>GLEALLRPKSIAVIGASMKPNRAGYLMMRNLLAGGFNGPVLPVTPAWKAVLGVLAWPDIASLPFTPDLAVLCTNASRNLALLEELGEKGCKTCIILSAPASQHEDLRACALRHNMRLLGPNSLGLLAPWQGLNASFSPVPIKRGKLAFISQSAAVSNTILDWAQQRKMGFSYFIALGDSLDIDVDELLDYLARDSKTSAILLYLEQLSDARRFVSAARSASRNKPILVIKSGRSPAAQRLLNTTAGMDPAWDAAIQRAGLLRVQDTHELFSAVETLSHMRPLRGDRLMIISNGAAPAALALDALWSRNGKLATLSEATCQKLRDALPEHVAISNPLDLRDDASSEHYIKTLDILLHSQDFDALMVIHSPSAAAPATESAQVLIEAVKHHPRSKYVSLLTNWCGEHSSQEARRLFSEAGLPTYRTPEGTITAFMHMVEYRRNQKQLRETPALPSNLTSNTAEAHLLLQQAIAEGATSLDTHEVQPILQAYGMNTLPTWIASDSTEAVHIAEQIGYPVALKLRSPDIPHKSEVQGVMLYLRTANEVQQAANAIFDRVKMAWPQARVHGLLVQSMANRAGAQELRVVVEHDPVFGPLIMLGEGGVEWRPEDQAVVALPPLNMNLARYLVIQGIKSKKIRARSALRPLDVAGLSQLLVQVSNLIVDCPEIQRLDIHPLLASGSEFTALDVTLDISPFEGDNESRLAVRPYPHQLEEWVELKNGERCLFRPILPEDEPQLQQFISRVTKEDLYYRYFSEINEFTHEDLANMTQIDYD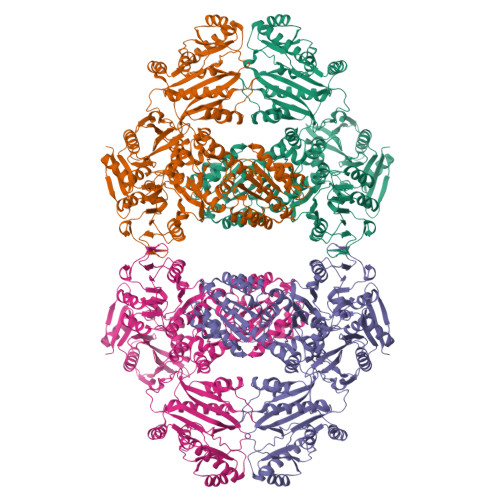REMAFVAVRRIDQTEEILGVTRAISDPDNIDAEFAVLVRSDLKGLGLGRRLMEKLITYTRDHGLQRLNGITMPNNRGMVALARKLGFNVDIQLEEGIVGLTLNLA[4x]>[2x]KNKVNRSFVDLGISTQRKIVYELYFAVKYLS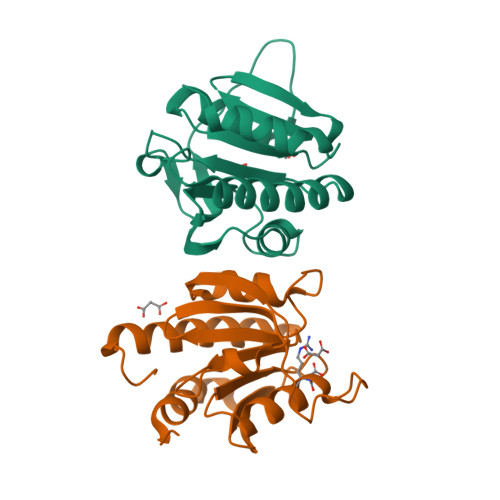KNKVGAIITLQRNILLDSLRTDGVKIDSLINSSLLIAIFQKSSPLHDGAVIIVDDRILYASTYFSVSESTLEDRYGARHRAALGISEVSDSITVVVSEQSGEVVIVRDANFFKVTNLETFTEVLTKELNSSQTNTAKKHHHHH>DGGARVGYIELDLNSGKVLESFRPEERFPMMSTFKVLLCGAVLSRI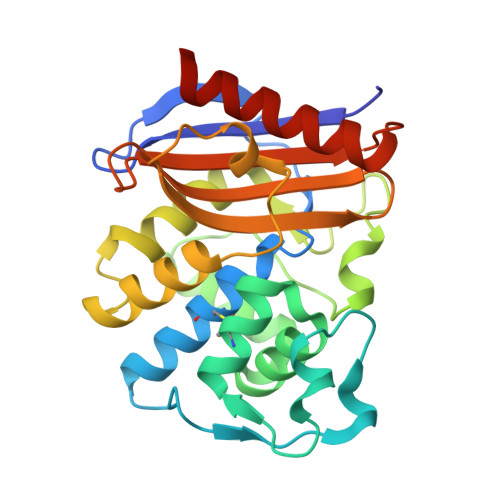DAGQEQLGRRIHYSQNDLVEYSPVTEKHLTDGMTVGELCSAAITMSDNTAANLLLTTIGGPKELTAFLHNMGDHVTRLDRWEPELNEAIPNDERDTTTPVAMATTLRKLLSGELLTLASRQQLMDWMEADKVAGPLLRSVLPAGWFIADKSGAGEHGSRGIIAALGPDGKPSRIVVIYMTGSQATMDERNRQIAEIGASLIGGHHHHH[2x]6-amino-2-({[(3a'R,4S,6'R,6a'R)-2,2,2',2'-tetramethyldihydro-3a'H-spiro[1,3-dioxolane-4,4'-furo[3,4-d][1,3]dioxol]-6'-yl]methyl}amino)-1,7-dihydro-8H-imidazo[4,5-g]quinazolin-8-one 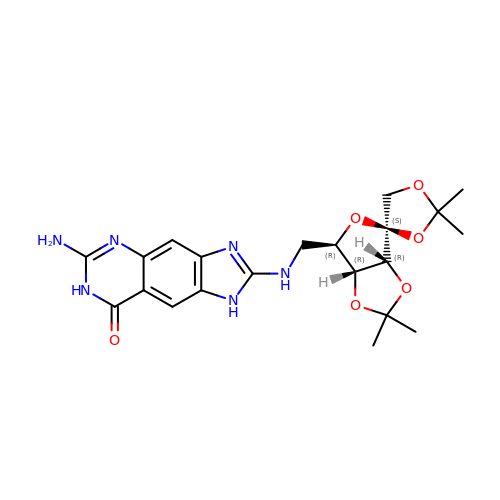(non-preferred name) | C21 H26 N6 O6 | SAAYEWUENSTOGT-JRMKUOIOSA-N Transient receptor potential melastatin 8 (TRPM8) channel is a Ca2+-permeable non-selective cation channel that acts as the primary cold sensor in humans. TRPM8 is also activated by ligands such as menthol, icilin, and phosphatidylinositol 4,5-bisphosphate (PIP2), and desensitized by Ca2+. MmTRPM8 is a homotetramer with dimensions of 140 × 110 × 110 Å. Each MmTRPM8 subunit contains multiple domains, including the N-terminal four TRPM homology repeats (MHR1 to MHR4), S1–S6 six transmembrane helices in a domain swap configuration, TRP helix, and C-terminal coiled-coil.

The ligand-free MmTRPM8 sample was obtained by adding 2 mM EGTA to chelate the trace amount of free Ca2+. The ligand-free state TRPM8 structure represents the full-length structure of mammalian TRPM8 channels with a canonical S4-S5 linker and the clearly resolved selectivity filter and outer pore loop. In MmTRPM8, the selectivity filter is lined by residues 912FGQ914. The backbone carbonyls of Phe912 and Gly913 along with the Gln914 side chain, build the ion conduction pathway with a minimum atom-to-atom diameter of ~9 Å between both Phe912 and Gly913 carbonyl oxygen atoms, suggesting the passage of hydrated ions during ion conduction. In the maps of MmTRPM8LMNG-ligand-free and MmTRPM8nanodisc-Ca-icilin-PIP2, but not others, sphere-shaped density peaks were clearly visible in the center of the selectivity and tentatively modeled as Na+ ions, the cation at the highest concentration in the sample. Distances between the putative Na+ and Gly913 carbonyl oxygens are ~4.5 Å, too far for direct ion coordination, supporting the passage of hydrated ions in the filter. In comparison, in the MmTRPM8 filter, the Gln914 side chain does not form a similar hydrogen bond with Gly913 carbonyl from its neighboring subunit and the atom-to-atom diameter is 1 Å larger than that in MmTRPM4. As Ca2+ has a larger hydration radius than K+ and Na+, the different filter diameters between MmTRPM8LMNG-ligand-free and MmTRPM4 may partially account for their difference in ion selectivity. In comparison, no density is observed at an equivalent site in the structure of MmTRPM8LMNG-ligand-free. The previously reported structure features in bird TRPM8 structures in the ligand-free state, such as low-resolution pore helix, invisible selectivity filter and outer pore loop, and one single straight helix formed by S4-S5 linker and S5, are not observed in the MmTRPM8 structure in the ligand-free state.

>MSFEGARLSMRSRRNGTMGSTRTLYSSVSRSTDVSYSDSDLVNFIQANFKKRECVFFTRDSKAMENICKCGYAQSQHIEGTQINQNEKWNYKKHTKEFPTDAFGDIQFETLGKKGKYLRLSCDTDSETLYELLTQHWHLKTPNLVISVTGGAKNFALKPRMRKIFSRLIYIAQSKGAWILTGGTHYGLMKYIGEVVRDNTISRNSEENIVAIGIAAWGMVSNRDTLIRSCDDEGHFSAQYIMDDFTRDPLYILDNNHTHLLLVDNGCHGHPTVEAKLRNQLEKYISERTSQDSNYGGKIPIVCFAQGGGRETLKAINTSVKSKIPCVVVEGSGQIADVIASLVEVEDVLTSSMVKEKLVRFLPRTVSRLPEEEIESWIKWLKEILESSHLLTVIKMEEAGDEIVSNAISYALYKAFSTNEQDKDNWNGQLKLLLEWNQLDLASDEIFTNDRRWESADLQEVMFTALIKDRPKFVRLFLENGLNLQKFLTNEVLTELFSTHFSTLVYRNLQIAKNSYNDALLTFVWKLVANFRRSFWKEDRSSREDLDVELHDASLTTRHPLQALFIWAILQNKKELSKVIWEQTKGCTLAALGASKLLKTLAKVKNDINAAGESEELANEYETRAVELFTECYSNDEDLAEQLLVYSCEAWGGSNCLELAVEATDQHFIAQPGVQNFLSKQWYGEISRDTKNWKIILCLFIIPLVGCGLVSFRKKPIDKHKKLLWYYVAFFTSPFVVFSWNVVFYIAFLLLFAYVLLMDFHSVPHTPELILYALVFVLFCDEVRQWYMNGVNYFTDLWNVMDTLGLFYFIAGIVFRLHSSNKSSLYSGRVIFCLDYIIFTLRLIHIFTVSRNLGPKIIMLQRMLIDVFFFLFLFAVWMVAFGVARQGILRQNEQRWRWIFRSVIYEPYLAMFGQVPSDVDSTTYDFSHCTFSGNESKPLCVELDEHNLPRFPEWITIPLVCIYMLSTNILLVNLLVAMFGYTVGIVQENNDQVWKFQRYFLVQEYCNRLNIPFPFVVFAYFYMVVKKCFKCCCKEKNMESNACCFRNEDNETLAWEGVMKENYLVKINTKANDNSEEMRHRFRQLDSKLNDLKSLLKEIANNIKLEGGSSGGWSHPQFEK[4x]>GNTTSSVILTNYMDTQYYGEIGIGTPPQTFKVVFDTGSSNVWVPSSKCSRLYTACVYHKLFDASDSSSYKHNGTELTLRYSTGTVSGFLSQDIITVGGITVTQMFGEVTEMPALPFMLAEFDGVVGMGFIEQAIGRVTPIFDNIISQGVLKEDVFSFYYNRDSENSQSLGGQIVLGGSDPQHYEGNFHYINLIKTGVWQIQMKGVSVGSSTLLCEDGCLALVDTGASYISGSTSSIEKLMEALGAKKRLFDYVVKCNEGPTLPDISFHLGGKEYTLTSADYVFQESYSSKKLCTLAIHAMDIP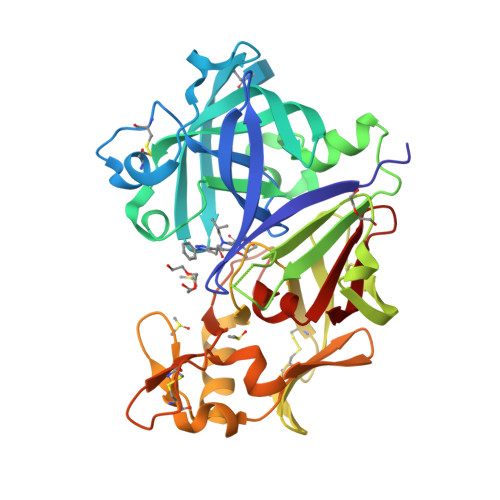PPTGPTWALGATFIRKFYTEFDRRNNRIGFALAR[2x]The Scribble (Scrib) protein is a conserved cell polarity regulator with anti-tumorigenic properties. Scribble is an important regulator of cell polarity and acts as a scaffolding protein to mediate a diverse set of cellular signalling pathways via its four PDZ domains. The zoonotic Tick-born encephalitis virus TBEV encodes for the NS5 protein, which has been shown to interact with Scribble in a PDZ domain dependent manner. In summary, we show that TBEV NS5 C-terminal PBM binds SCRIB PDZ3 in order to interact with Scribble.

To understand the interactions of SCRIB PDZ domain interactions with NS5 PBM sequences in more detail we determined crystal structures of SCRIB PDZ3:NS5_CTN complexes as well as a structure of SCRIB PDZ3 apo. Unexpectedly, when determining the crystal structure of the SCRIB PDZ3:NS5_CTN complex we observed a heterotrimer with a 2 : 1 stoichiometry comprising only a single NS5_CTN chain. The complex of SCRIB PDZ3:NS5_CTN revealed an unexpected stoichiometry, where a single NS5_CTN peptide was bound in an antiparallel manner in the canonical PDZ binding groove of a single SCRIB PDZ3 molecule (Chain A), with a second SCRIB PDZ3 molecule (Chain B) engaging the same peptide via its β2 strand. In this 2:1 complex an extended β-sheet between Chain A β2-NS5_CTN-Chain B β2 is formed. Examination of the SCRIB PDZ3 molecule engaging NS5_CTN using the canonical ligand binding groove reveals that eight hydrogen bonds are formed upon binding, including a double bond between Ser3412NS5–Ile1018PDZ3, and single bonds with Ile3414NS5–Leu1014PDZ3, Ile3414NS5–Gly1015PDZ3, Ile3414NS5–Leu1016PDZ3, Glu3410NS5–Gln1072PDZ3 and Ile3409NS5–His1023PDZ3 as well as Ser3412NS5–His1071PDZ3. The non-canonical interaction between a second SCRIB PDZ3 domain and NS5_CTN involves two hydrogen bonds with Ile3413NS5–Leu1016PDZ3 and Ser3412NS5–Ile1018PDZ3, as well as a single bond between Glu3410NS5–Ser1039PDZ3 at β3 and Ser3411NS5–His1071PDZ3. Interesting, Glu3410NS5 is able to contact Gln1072PDZ3 whereas in the PDZ3: β-PIX complex the equivalent Asp642β-PIX is too short to reach Gln1072PDZ3. The Ser1039PDZ3–Glu643β-PIX interaction is recapitulated in a more unconventional configuration, with the Ser1039PDZ3 being provided by chain B which binds NS5 in a non-canonical manner. Previously SCRIB PDZ3 had only been shown to form 1 : 1 heterodimers with PBM peptides via the canonical PDZ binding groove. Examination of the SCRIB PDZ3:NS5_CTN interaction using ITC demonstrated a 1 : 1 stoichiometry, suggesting that the binding of the second protomer in a non-canonical manner is likely due to crystallographic packing and not biologically relevant.

>[2x]SVEEIRLPRAGGPLGLSIVGGSDHSSHPFGVQEPGVFISKVLPRGLAARSGLRVGDRILAVNGQDVRDATHQEAVSALLRPCLELSLLVRRD;> LRLESSII> MTENILRKSDEEIQKEITARVKALESMLIEQGILTTSMIDRMAEIYENEVGPHLGAKVVVKAWTDPEFKKRLLADGTEACKELGIGGLQGEDMMWVENTDEVHHVVVCTLCSCYPWPVLGLPPNWFKEPQYRSRVVREPRQLLKEEFGFEVPPSKEIKVWDSSSEMRFVVLPQRPAGTDGWSEEELATLVTRESMIGVEPAKAV;> MNGVYDVGGTDGLGPINRPADEPVFRAEWEKVAFAMFPATFRAGFMGLDEFKFGIEQMNPAEYLESPYYWHWIRTYIHHGVRTGKIDLEELERRTQYYR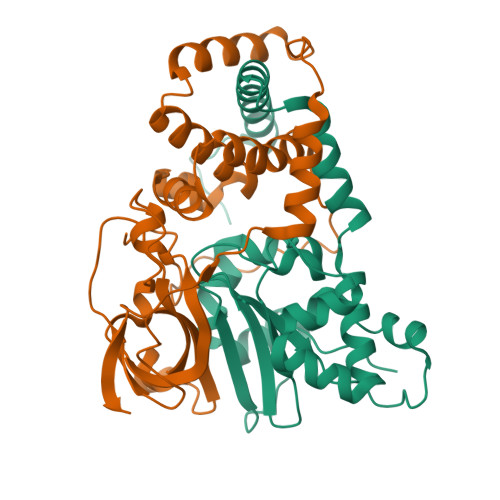ENPDAPLPEHEQKPELIEFVNQAVYGGLPASREVDRPPKFKEGDVVRFSTASPKGHARRARYVRGKTGTVVKHHGAYIYPDTAGNGLGECPEHLYTVRFTAQELWGPEGDPNSSVYYDCWEPYIELVDT> RAVPGGSSPAWTQCQQLSQKLCTLAWSA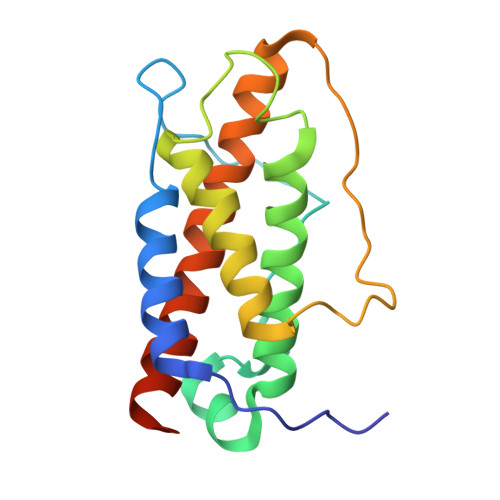HPLVGHMDLREEGDEETTNDVPHIQCGDGCDPQGLRDNSQFCLQRIHQGLIFYEKLLGSDIFTGEPSLLPDSPVGQLHASLLGLSQLLQPEGHHWETQQIPSLSPSQPWQRLLLRFKILRSLQAFVAVAARVFAHGAATLSPGSHHHHHH> GICKSSDCIKSAARLIQNMDATTEPCTDFFKYACGGWLKRNVIPETSSRYGNFDILRDELEVVLKDVLQEPKTEDIVAVQKAKALYRSCINESAIDSRGGEPLLKLLPDIYGWPVATENWEQKYGASWTAEKAIAQLNSKYGKKVLINLFVGTDDKNSVNHVIHIDQPRLGLPSRDYYECTGIYKEACTAYVD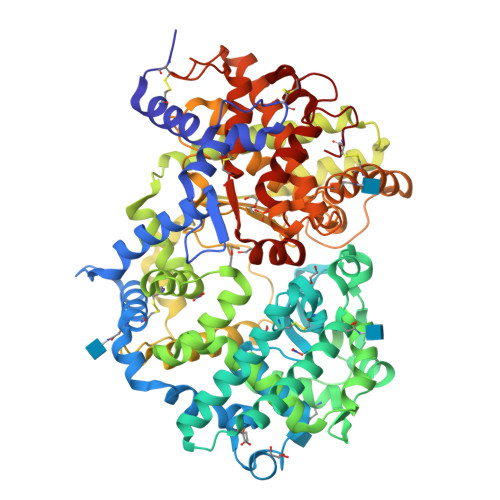FMISVARLIRQEERLPIDENQLALEMNKVMELEKEIANATAKPEDRNDPMLLYNKMTLAQIQNNFSLEINGKPFSWLNFTNEIMSTVNISITNEEDVVVYAPEYLTKLKPILTKYSARDLQNLMSWRFIMDLVSSLSRTYKESRNAFRKALYGTTSETATWRRCANYVNGNMENAVGRLYVEAAFAGESKHVVEDLIAQIREVFIQTLDDLTWMDAETKKRAEEKALAIKERIGYPDDIVSNDNKLNNEYLELNYKEDEYFENIIQNLKFSQSKQLKKLREKVDKDEWISGAAVVNAFYSSGRNQIVFPAGILQPPFFSAQQSNSLNYGGIGMVIGHEITHGFDDNGRNFNKDGDLVDWWTQQSASNFKEQSQCMVYQYGNFSWDLAGGQHLNGINTLGENIADNGGLGQAYRAYQNYIKKNGEEKLLPGLDLNHKQLFFLNFAQVWCGTYRPEYAVNSIKTDVHSPGNFRIIGTLQNSAEFSEAFHCRKNSYMNPEKKCRVW> AAPPVQSQVDCENSQPWHVAVYRFNKYQCGGVLLDRNWVLTAAHCYNDKYQVWLGKNNFLEDEPSDQHRLVSKAIPHPDFNMSLLNEHTPQPEDDYSNDLMLLRLSKPADITDVVKPITLPTEEPKLGSTCLASGWGSTTPIKFKYPDDLQCVNLKLLPNEDCDKAHEMKVTDAMLCAGEMDGGSYTCEHDSGGPLICDGI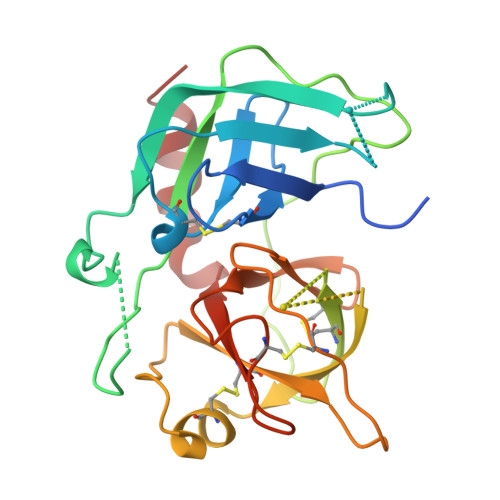LQGITSWGPEPCGEPTEPSVYTKLIKFSSWIRETMANNP An important bacterial virulence factor is the secreted serine protease HtrA (HtrACj), which targets tight and adherens junctional proteins in the gut epithelium. A characteristic feature of the HtrA family of proteins is the presence of a chymotrypsin-type protease domain as well as one or two C-terminal PDZ domains (Postsynaptic density protein 95, Drosophila disc large tumor suppressor and Zonula occludens-1 protein domain). We have demonstrated that C. jejuni HtrA is a periplasmic protein, but it can also be secreted into the extracellular environment. Extracellular HtrACj is involved in virulence as it cleaves the adherens junction protein E-cadherin, an important factor required for maintaining an intact epithelial barrier.

Since the proteolytically active HtrACj wild-type revealed a high tendency to auto-proteolysis, we expressed a proteolytically inactive recombinant S197A substitution mutant of HtrACj in E. coli, and after purification of the protein, the structure was investigated by Cryo-EM. Data analysis produced a 3D map at 5.8 Å resolution. HtrACj monomers have an elongated, bent shape with three well-separated structural domains (I–III): a central core domain that is responsible for the chymotrypsin-like protease (N-terminus up to residue 273) and two joining PDZ domains, PDZ1 (residues 275–362) and PDZ2 (residues 376–471). The basic unit of the structural organization of HtrACj is the trimer, with three monomers arranged around a three-fold axis. The three monomers interact via their proteolytic domains, whilst the two PDZ domains radiate outwards. In the higher-order assembly, four trimers of HtrACj arrange into a dodecamer, characterized by a tetrahedral symmetry, consisting of 4 threefold rotation axes, running from each vertex of the tetrahedron to the center of an opposite face, and 3 twofold axes, running from the middle of each edge to the middle of an opposite edge. The contacts between trimers in the dodecamer are quite loose, as the trimers are only held together by interactions between three PDZ2 domains of one trimer and the three PDZ1 domains of the other three trimers. Within each trimer, there is a small gap that may be permeable only to solvent molecules, whilst the gap on the opposite side of the dodecameric assembly is quite large, being a triangular aperture of about 36 Å from a vertex to an edge. Six large rectangular openings of about 32 Å x 24 Å are also present in correspondence of the 3 twofold axes. The buried surface area following the formation of the dodecamer in HtrACj is significantly smaller, leading to a significantly less stable and more flexible assembly.

>VLSYHDSIKDAKKSVVNISTSKTITRANRPSPLDDFFNDPYFKQFFDFDFPQRKGKNDKEVVSSLGSGVIISKDGYIVTNNHVVDDADTITVNLPGSDIEYKAKLIGKDPKTDLAVIKIEANNLSAITFTNSDDLMEGDVVFALGNPFGVGFSVTSGIISALNKDNIGLNQYENFIQTDASINPGNSGGALVDSRGYLVGINSAILSRGGGNNGIGFAIPSNMVKDIAKKLIEKGKIDRGFLGVTILALQGDTKKAYKNQEGALITDVQKGSSADEAGLKRGDLVTKVNNKVIKSPIDLKNYIGTLEIGQKISLSYERDGENKQASFILKGEKENPKGVQSDLIDGLSLRNLDPRLKDRLQIPKDVNGVLVDSVKEKSKGKNSGFQEGDIIIGVGQSEIKNLKDLEQALKQVNKKEFTKVWVYRNGFATLLVLK[12x]> YLNIFISHHEVMKLMGLEADLFYVHEGAINTYAMHFTVPVPADVHELEFSWQSLIA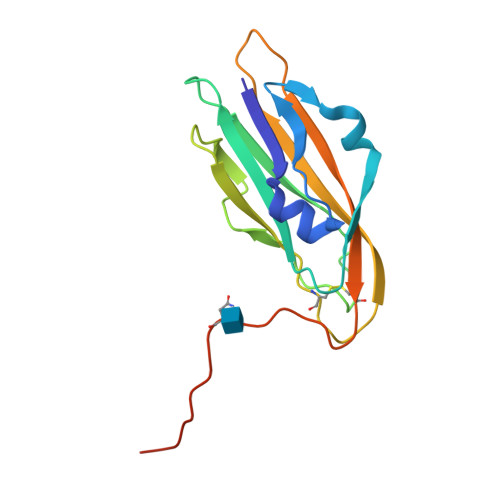YPLPYAISIEYNNDQEALGTPTLSIPHKGLVPQEIESFLVYLPCTGNASLQMPVNVNMVVRAPPRFNDTRLHFKRNKICAKGISPEPNQSPAPAHAPSQGPAIEGR> TSTKRFTCPEESEASNCSCEEFPSKTHFYCPDFNPTLYVDVEDRMRVDFKCYDEPHDFKSLPNLAIGSVKLLTVVDCVLDDDRPILESFKFLEVADVRSFVYNNHENGIRYNAKYFEGMEQLENLTLARGVVSIDRDTFSGFLNLKRLTIEHNKLNLQPGTFEALSNLTYLGLVYNGLNEIQPGLFDGLESLEALSLSYNDIKSLSAGSFNGLSSLRMLNLRVNKIESFDANTFASLKELSRLEITLNPF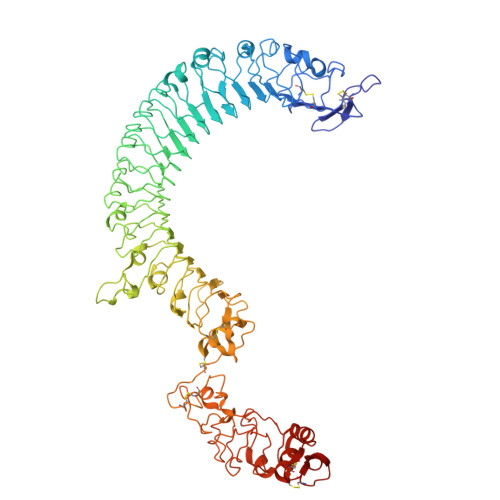VSLPRGLFSENKKLKTLILTNNRKLVTLPEELLANLKELTVVNLSHNGVGNLPESLLSGSSGIIELNLGYNRLNSLPEELLSDQPQLQVLNLDHNQLESIPDYFLERNVELQTLYLSHNRLRSLSEKAFTKLKNLKELHLENNQLQTIPQFLFSGTPKLEEIYMQNNQLALHANSFINEELSIADNDNTPFQVLQKLRILHLRNNSISTIFQDWYINNLEMQSLDLSFNKLPGLSYTQLQFQSNITLNLSNNEISQVLLIDDLDLQPYQRINVDLNHNPLNCNCNALKFIQLIQSKAEHGLQFNVDQLRCSEPPNLLDATMDQLQTKDLLCDFESADDCPKDCQCAMRLLDHTVIVNCSGRGLTEFPDLPIPSQLHEDFNALEVHVENNRLTKLPNLTKHNEITQLYARNNSIQNLLPHNIPSKLRIIDLSQNLLKMIDDSTLAQINRSSHLETIRLSQNQWLCDCPASSFLIFVQQNSRLISDMSAIRCHPSGKSLDSITVNELCFEDYTTENLYFQ>PFVNKQFNYKDPVNGVDIAYIKIPNAGQMQPVKAFKIHNKIWVIPERDTFTNPEEGDLNPPPEAKQVPVSYYDSTYLSTDNEKDNYLKGVTKLFERIYSTDLGRMLLTSIVRGIPFWGGSTIDTELKVIDTNCINVIQPDGSYRSEELNLVIIGPSADIIQFECKSFGHEVLNLTRNGYGSTQYIRFSPDFTFGFEESLEVDTNPLLGAGKFATDPAVTLAHELIHAGHRLYGIAINPNRVFKVNTNAYYEMSGLEVSFEELRTFGGHDAKFIDSLQENEFRLYYYNKFKDIASTLNKAKSIVGTTASLQYMKNVF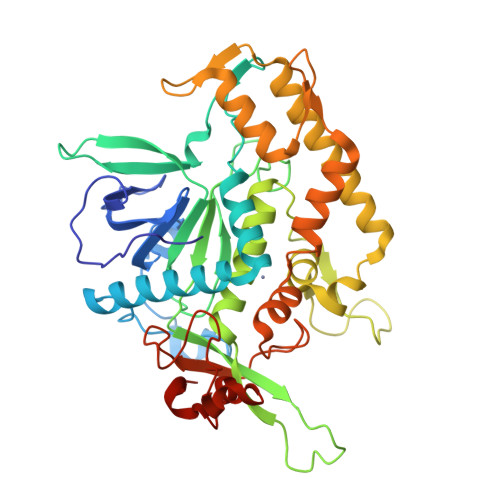KEKYLLSEDTSGKFSVDKLKFDKLYKMLTEIYTEDNFVKFFKVLNRKTYLNFDKAVFKINIVPKVNYTIYDGFNLRNTNLAANFNGQNTEINNMNFTKLKNFTPG[2x]>[2x]M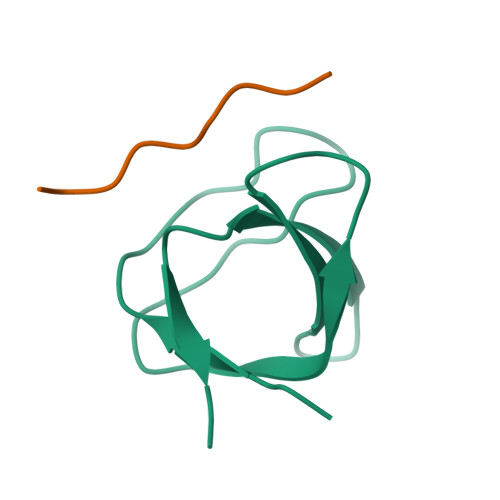VDYIVEYDYDAVHDDELTIRVGEIIRNVKKLQEEGWLEGELNGRRGMFPDNFVKEIKRETE;>KGPPLPRPRV[2x]> APASIDWRKKGAVTSVKDQGA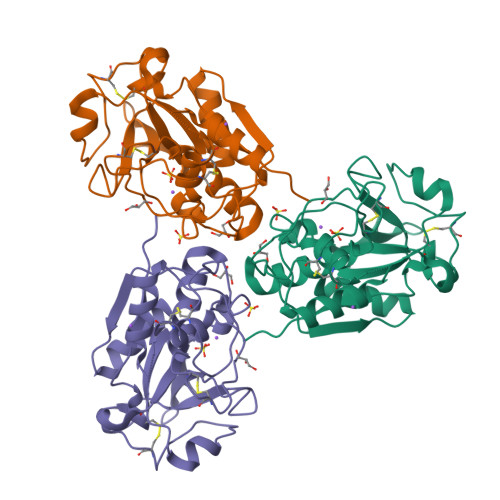CGMCWAFGATGAIEGIDAITTGRLISVSEQQIVDCDTXXXXXXGGDADDAFRWVITNGGIASDANYPYTGVDGTCDLNKPIAARIDGYTNVPNSSSALLDAVAKQPVSVNIYTSSTSFQLYTGPGIFAGSSCSDDPATVDHTVLIVGYGSNGTNADYWIVKNSWGTEWGIDGYILIRRNTNRPDGVCAIDAWGSYPTKSTS(2~{R},6~{S})-2,6-diacetamido-7-[[(2~{R})-1-(oxidanylamino)-1-oxidanylidene-propan-2-yl]amino]-7-oxidanylidene-heptanoic 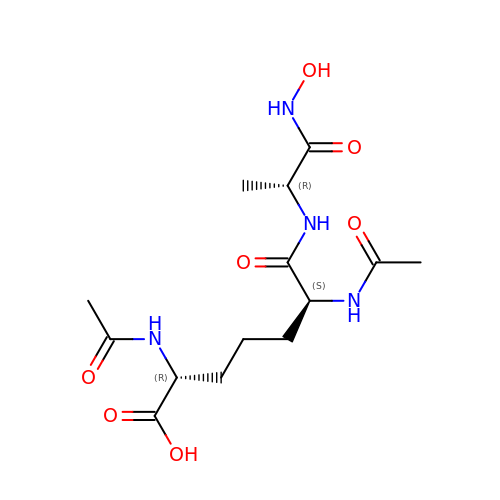acid | C14 H24 N4 O7 | OVQLZBDGLZLNSO-PPKCKEKNSA-N> SMA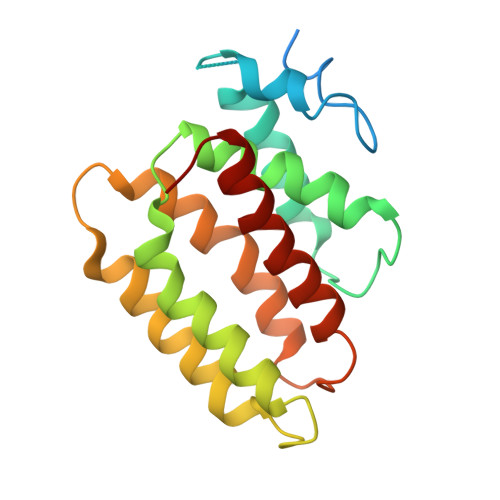YHQKHGGYGRGGYGRQDRPQVDASRLFGESPDVVGIKKMLEGKGKQWEAIQPYFDNVVREAKNFLEWSPNKRLANAVTVAAYLTSQGLKTNQVRKILDMARTTELKVKRGEGDIKDDLVKMRYLLAYTVGKATGQSKYSLDAFHRILDPMLEVLMGSPKKENFEKFYDFLQAVVAYHKFFGGGD>[6x]MANCERTFIAIKPDGVQRGLVGEIIKRFEQKGFRLVGLKFMQASEDLLKEHYVDL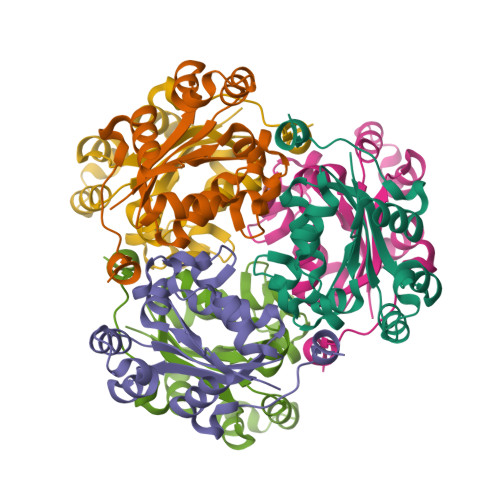KDRPFFAGLVKYMHSGPVVAMVWEGLNVVKTGRVMLGETNPADSKPGTIRGDFCIQVGRNIIHGSDSVESAEKEIGLWFHPEELVDYTSCAQNWIYE N-(4-{[(2-amino-4-hydroxyquinazolin-6-yl)methyl](formyl)amino}benzoyl)-L-glutamic acid | C22 H21 N5 O7 | 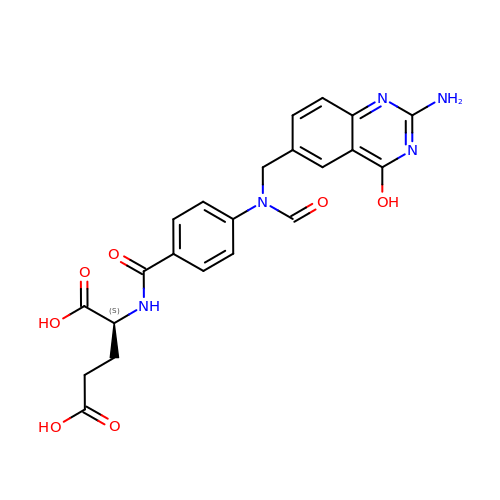QHUBQNFYSLRYQG-KRWDZBQOSA-N> ADTCYNDVALDCGITSNSLALPRCNAVYGEYGSHGNVATELQAYAKLHLERSYDYLLSAAYFNNYQTNRAGFSKLFKKLSDEAWSKTIDIIKHVTKRGDKMNFDQH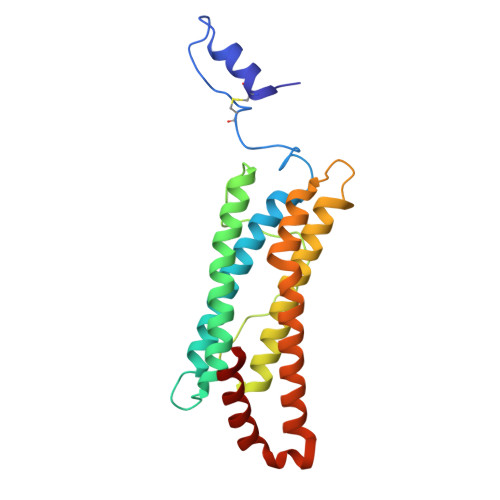STMKTERKNYTAENHELEALAKALDTQKELAERAFYIHREATRNSQHLHDPEIAQYLEEEFIEDHAEKIRTLAGHTSDLKKFITANNGHDLSLALYVFDEYLQKTV>GTGPDKLKKVLDKLRLKRKDISEAAETVNKVVERLLRRMQKRESEFKGVEQLNTGSYYEHVKISAPNQFNVMFKLEVPRIELQEYYETGAFYLVKFKRIPRGNPLSHFLEGEVLSATKMLSKFRKIIKEEVKEIKDIDVSVEKEKPGSPAVTLLIRNPEEISVDIILALESKGSWPISTKEGLPIQGWLGTKVRTNLRREPFYLVPKNAKDGNSFQGETWRLSFSHTEKYILNNHGIEKTCCESSGAKCCRKECLKLMKYLLEQLKKEFQELDAFCSYHVKTAIFHMWTQDPQDSQWDPRNLSSCFDKLLAFFLECLRTEKLDHYFIPKFNLFSQELIDRKSKEFLSKKIEYERNNGFPIFDKL[2x]

Cyclic GMP-AMP (cGAMP) synthase (cGAS) is essential for the host defense against cytosolic double-stranded (ds)DNA arising from various maladies (e.g., pathogen invasion, ionizing irradiation, and genotoxic chemicals). Upon directly binding to and dimerizing on dsDNA, cGAS cyclizes ATP and GTP into 2′−5′/3′−5′-linked cGAMP, a unique metazoan second messenger for initiating type-I interferon (IFN-I)-mediated inflammatory responses. cGAS is central to antitumor immunity, host defense against an array of pathogens, and regulating autoimmunity. Here, we resolve these numerous fundamental mechanistic questions in innate immunology and present a unifying catalytic mechanism of cGAS. Finally, we reveal how mouse cGAS achieves more stringent substrate selectivity and higher catalytic efficiency than the human enzyme. Together, we set forth a unifying catalytic mechanism of cGAS in which dsDNA-binding pre-organizes the active site into a rigid yet adaptable lock for two sets of keys (substrates and intermediate) necessary to specifically synthesize 2′−5/3′−5′-cGAMP.

To test functional implications, we soaked QN-mcGAScat•dsDNA with inosine triphosphate (ITP)/GTP or ATP/ITP. Moreover, the ATP/ITP-soaked structure suggested that ATP and ITP are bound at Site-1 and Site-2, respectively; the carboxyl oxygen of ITP appeared to accept a H-bond from Ser366 as seen from GTP, and ATP fails to bind stably at Site-2 in all known structures (see also below for the pppGpA-bound structure). These results support the idea that the -NH2 of GTP is disfavored at Site-1 while the -NH2 of ATP at Site-1 provides a favorable interaction for site-specific ATP/GTP binding. E, F QN-mcGAScat•dsDNA bound to ITP/GTP (E) and ATP/ITP (F).> ANCRILLTPLNERDEQRGYSTQGLKRLSGTAKLNPRLGFTR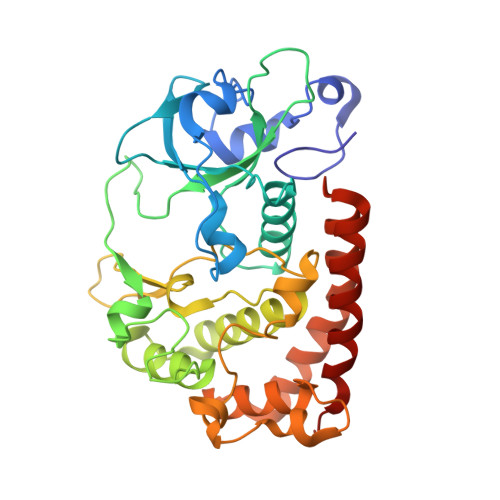TQFVQELPRQQKGMSIAGYQPKLQLVLDEGEFRVVDHQGNFILKPSPADFPGLAENEHATMTLMSRLGFDVPVHGLLSFAPQSEEELEYAFVIRRYDRDNKGLPVHQEQLDGAMQITDKYGKTGNDNEQYVSYETLARFLVAHVNDNIAFKIDLFRRIVYAWLLGNNDMHLRNFGLVYSDGLTPALAPVYDFVSVAPYPEYFYSNYLALPLLTREEGGRELAPGFHSDYGEYIGQDFLLLGESMGLAPRLLEKLFQDIRKENAIVMETYEQSFMTQDHIQAVLQCYRHRLGLLHHHHHH> AMSRSRPELGDWSSPAELAELQRSQLPRVLAQALRSPFYAARYRGTTPPRTADDFAGVEVTAKQDLRDQYPFGMLAVGREHLATYHESSGTAGEPTASYYTEEDWTDLAERFARKWTGIHPSDTFLVRTPYGLVITGHLAQAAGRLRGATVVPGDARSLATPLSRMVRVLKTLDVTLTWCNPTEITMLAAAAKAAGLRPDQDFPHLRAMFTAAEPLTEVRRRRLSEIWGGIPVVEEYGSTETGTIAGQCP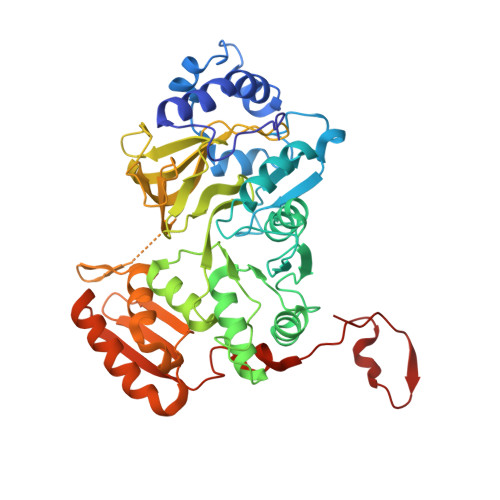EGRMHLWADRAIFEVYDPRTGTLSEAGRGQMVVTPLYRDAMPLLRYNLADDVEVSTDPCGCGWLLPTVTVLGRAGTGHRIGPATVTQQRLEELVFSLPAAYEVMFWRAKAHPDVLELEFEAPEPVRQRAVKELGAALDRELGVPHRITGLAPGTLVPAEALTAQRDILKARYLFAEDEDWDKAVMYF> VAQLTIGNSTITTQEAANIIVGYGEWPSYCSDSDATAVDKPTRPDVSVNRFYTLDTKLWEKSSKGWYWKFPDVLTETGVFGQNAQFHYLYRSGFCIHVQCNASKFHQGALLVAVLPEYVIGTVAGGTGTEDTHPPYKQTQPGADGFELQHPYVLDAGIPISQLTVCPHQWINLRTNNCATIIVPYINALPFDSALNHCNFGLLVVPISPLD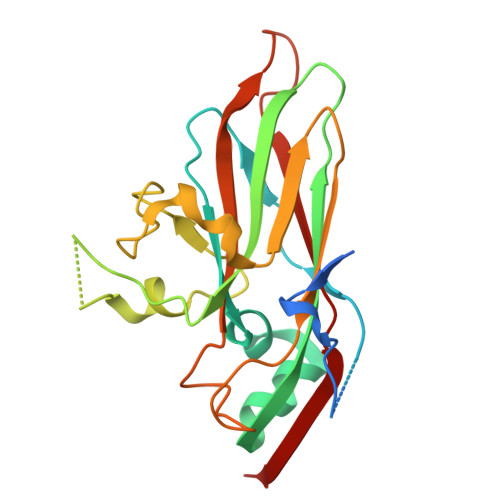YDQGATPVIPITITLAPMCSEFAGLR>GHMVSCSAPGKIYLFGEHAVVYGETAIACAVELRTRVRAELNDSITIQSQIGRTGLDFEKHPYVSAVIEKMRKSIPINGVFLTVDSDIPVGSGLGSSAAVTIASIGALNELFGFGLSLQEIAKLGHEIEIKVQGAASPTDTYVSTFGGVVTIPERRKLKTPDCGIVIGDTGVFSSTKELVANVRQLRESYPDLIEPLMTSIGKISRIGEQLVLSGDYASIGRLMNVNQGLLDALGVNILELSQLIYSARAAGAFGAKITGAGGGGCMVALTAPEKCNQVAEAVAG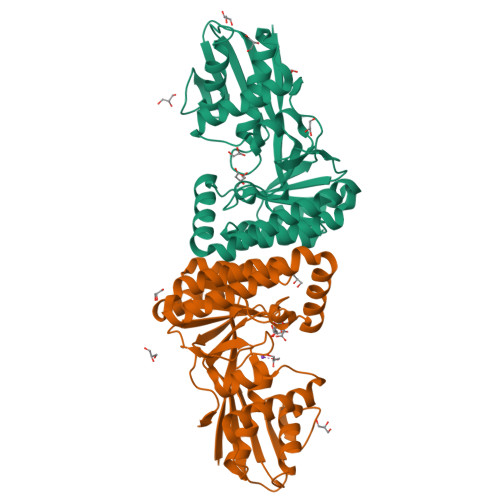AGGKVTITKPTEQGLKVD[2x]>[4x]GMRQRDDSKRIAFLEATVREVADHGFSATSVGKIAKAAGLSPATLYIYYEDKEQLLLATFYYVSDQVIDAALDSFSRGKDLREGLRRQWHTLFRIGLERPEL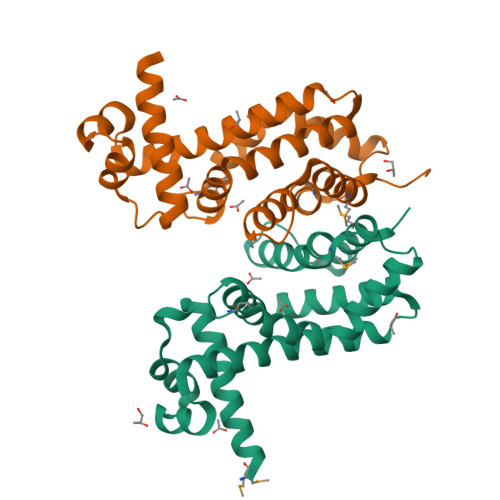FRYHETFTHSAWMTPEIQARNESRAANLLNAVDQGKQSGLIKPVPFPLLETFMFRPIYHLVQRCLQGSFEGTDEHIELAFNMAWDAVADRRNT>[2x]MDHLPIFCQLRDRDCLIVGGGDVAERKARLLLEAGARLTVNALTFIPQFTVWANEG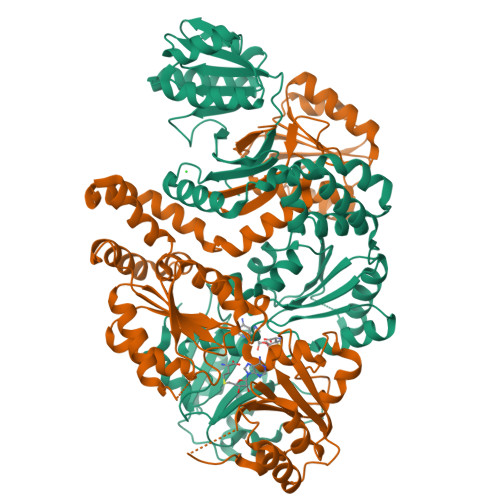MLTLVEGPFDETLLDSCWLAIAATDDDTVNQRVSDAAESRRIFCNVVDAPKAASFIMPSIIDRSPLMVAVSAGGTSPVLARLLREKLESLLPQHLGQVARYAGQLRARVKKQFATMGERRRFWEKFFVNDRLAQSLANADEKAVNATTERLFSEPLDHRGEVVLVGAGPGDAGLLTLKGLQQIQQADIVVYDRLVSDDIMNLVRRAADRVFVGKRAGYHCVPQEEINQILLREAQKGKRVVRLKGGDPFIFGRGGEELETLCHAGIPFSVVPGITAASGCSAYSGIPLTHRDYAQSVRLVTGHLKTGGELDWENLAAEKQTLVFYMGLNQAATIQEKLIAFGMQADMPVALVENGTSVKQRVVHGVLTQLGELAQQVESPALIIVGRVVALRDKLNWFSNH The mer operons are under the regulation of the mercury(II)-dependent transcriptional repressor-activator MerR. Thus, in the absence of mercury(II), MerR still represses the transcription of the structural genes by capturing RNA polymerase in a closed inactive state. Upon mercury(II) binding, the conformation changes of MerR induce a local underwinding of the promoter DNA, which facilitates the formation of an open complex by RNA polymerase to initiate transcription. MerR is a representative metalloregulatory protein that exhibits high sensitivity and selectivity to mercury(II) in vivo and in vitro.

Here we report the crystal structure of the C-terminally truncated Tn501 MerR in complex with mercury(II). The mercury(II)-bound Tn501 MerR was crystallized as a functional dimer in an asymmetrical unit of the P3121 space group. Each monomer contains three distinct functional domains comprising an N-terminal DNA-binding domain (DBD, residues 1–81), a C-terminal metal-binding domain (CBD, residues 119–134), and an amphipathic dimerization helix (DH, residues 82–118). The long dimerization helix plays a critical role in stabilizing the dimer by the formation of an antiparallel coiled-coil dimer interface. In the functional dimer of Tn501 MerR, there are two mercury ions bound at the equivalent site. However, only one metal-binding loop in the MerR dimer is fully ordered. In Tn501 MerR, the bounded mercury(II) shows planar trigonal coordination geometry with the S-atoms from three conserved cysteine residues (Cys82, Cys117, and Cys126). The Hg–S bond length in the mercury(II)-cysteine complex is consistent at ~2.56 Å, and the largest S-Hg-S angle is at 127°. The angular deviation from the perfect 120° may be caused by a steric effect derived from the pyrrolidine of Pro127, which is packed above the Hg-SCys117 and Hg-SCys126 bonds. The Gly79 residue in the corresponding hinge region participates in hydrogen-bonding interactions not only with residues Ser125′and Cys126′ of the metal-binding domain from the other monomer, but also with residue Glu77 adjacent to the C-terminus of the α4-helix.

>[2x]MENNLENLTIGVFAKAAGVNVETIRFYQRKGLLLEPDKPYGSIRRYGEADVTRVRFVKSAQRLGFSLDEIAELLRLEDGTHCEEASSLAEHKLKDVREKMADLARMEAVLSELVCACHARRGNVSCPLIASLQG> MAFCIAVIGKDNAPLYLTTSDMEQELELQYHV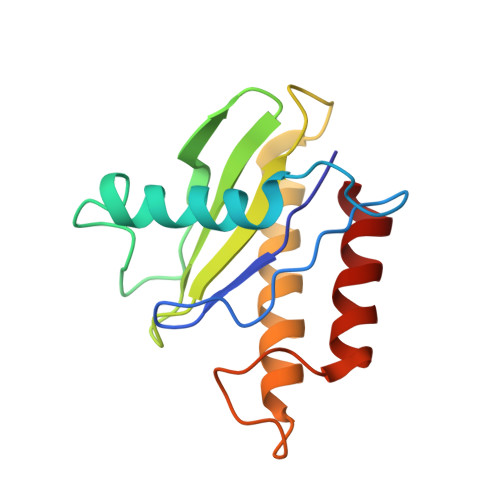NAALDVVEEKCLIGKGAPESKELYLGLLYSTENHKIYGFVTNTRVKFIVVIDSSNVALRENEVRAIFRNLHLLYTDAICNPFYIPGESLTSKKFDRAVQKLMSGTA>[2x]GHMEQTS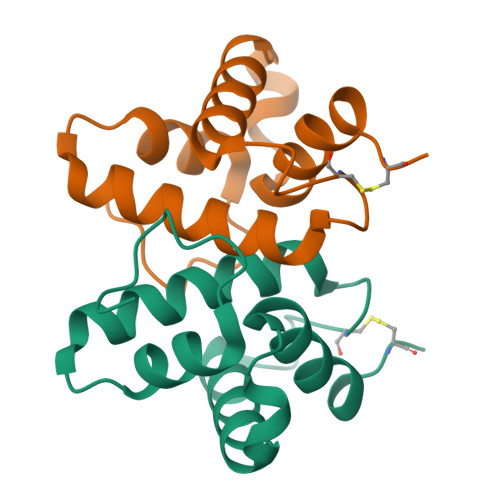IAHLTSDDVNLPGSDFFRFYRSADKQEKEKARIYLLGVLDATEGKSWCQYSQLQTVTLQEFVFEFFNKLPAARLHERAAPLIEEALATRFPCKGGKA> EENFSRSYPCDEKKQNDSVIAECSNRRLQEVPQTVGKYVTELDLSDNFITHITNESFQGLQNLTKINLNHNPNVQHQNGNPGIQS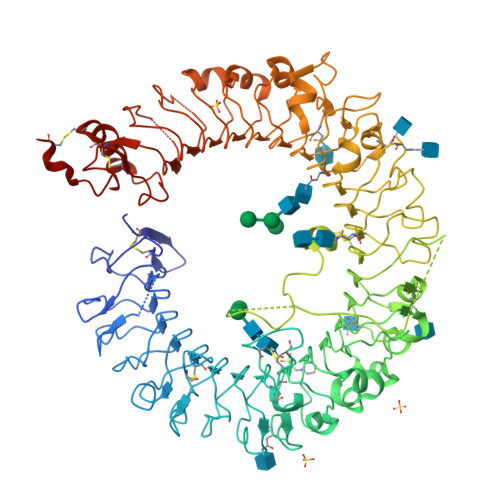NGLNITDGAFLNLKNLRELLLEDNQLPQIPSGLPESLTELSLIQNNIYNITKEGISRLINLKNLYLAWNCYFNKVCEKTNIEDGVFETLTNLELLSLSFNSLSHVPPKLPSSLRKLFLSNTQIKYISEEDFKGLINLTLLDLSGNCPRCFNAPFPCVPCDGGASINIDRFAFQNLTQLRYLNLSSTSLRKINAAWFKNMPHLKVLDLEFNYLVGEIASGAFLTMLPRLEILDLSFNYIKGSYPQHINISRNFSKLLSLRALHLRGYVFQELREDDFQPLMQLPNLSTINLGINFIKQIDFKLFQNFSNLEIIYLSENRISPLVKDTRQSYANSSSFQRHINQSNSTDFEFDPHSNFYHFTRPLIKPQCAAYGKALDLSLNSIFFIGPNQFENLPDIACLNLSANSNAQVLSGTEFSAIPHVKYLDLTNNRLDFDNASALTELSDLEVLDLSYNSHYFRIAGVTHHLEFIQNFTNLKVLNLSHNNIYTLTDKYNLESKSLVELVFSGNRLDILWNDDDNRYISIFKGLKNLTRLDLSLNRLKHIPNEAFLNLPASLTELHINDNMLKFFNWTLLQQFPRLELLDLRGNKLLFLTDSLSDFTSSLRTLLLSHNRISHLPSGFLSEVSSLKHLDLSSNLLKTINKSALETKTTTKLSMLELHGNPFECTCDIGDFRRWMDEHLNVKIPRLVDVICASPGDQRGKSIVSLELTTCVSDVT6-~{tert}-butylsulfonyl-~{N}-(3,4-dimethyl-1~{H}-pyrazol-5-yl)-7-methoxy-quinolin-4-amine | 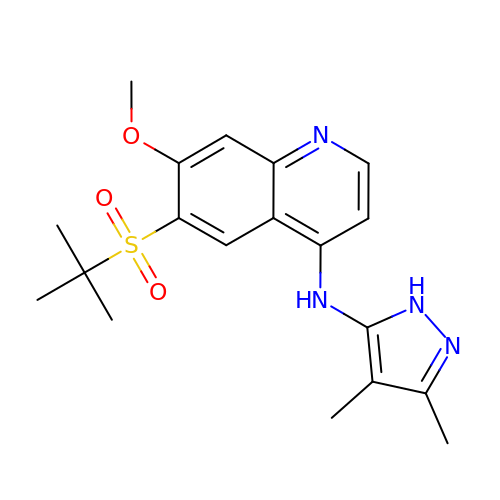C19 H24 N4 O3 S | LHPFRDAGGDMRMZ-UHFFFAOYSA-N> MELENYKQPVVLREDNCRRRRRMKPR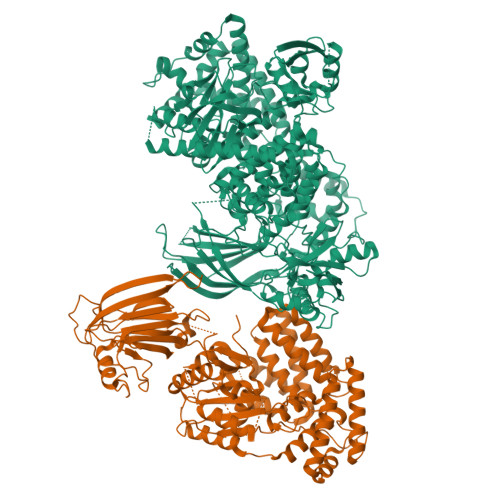SAAASLSSMELIPIEFVLPTSQRKCKSPETALLHVAGHGNVEQMKAQVWLRALETSVAADFYHRLGPHHFLLLYQKKGQWYEIYDKYQVVQTLDCLRYWKATHRSPGQIHLVQRHPPSEESQAFQRQLTALIGYDVTDVSNVHDDELEFTRRGLVTPRMAEVASRDPKLYAMHPWVTSKPLPEYLWKKIANNCIFIVIHRSTTSQTIKVSPDDTPGAILQSFFTKMAKKKSLMDIPESQSEQDFVLRVCGRDEYLVGETPIKNFQWVRHCLKNGEEIHVVLDTPPDPALDEVRKEEWPLVDDCTGVTGYHEQLTIHGKDHESVFTVSLWDCDRKFRVKIRGIDIPVLPRNTDLTVFVEANIQHGQQVLCQRRTSPKPFTEEVLWNVWLEFSIKIKDLPKGALLNLQIYCGKAPALSSKASAESPSSESKGKVQLLYYVNLLLIDHRFLLRRGEYVLHMWQISGKGEDQGSFNADKLTSATNPDKENSMSISILLDNYCHPIALPKHQPTPDPEGDRVRAEMPNQLRKQLEAIIATDPLNPLTAEDKELLWHFRYESLKHPKAYPKLFSSVKWGQQEIVAKTYQLLARREVWDQSALDVGLTMQLLDCNFSDENVRAIAVQKLESLEDDDVLHYLLQLVQAVKFEPYHDSALARFLLKRGLRNKRIGHFLFWFLRSEIAQSRHYQQRFAVILEAYLRGCGTAMLHDFTQQVQVIEMLQKVTLDIKSLSAEKYDVSSQVISQLKQKLENLQNSQLPESFRVPYDPGLKAGALAIEKCKVMASKKKPLWLEFKCADPTALSNETIGIIFKHGDDLRQDMLILQILRIMESIWETESLDLCLLPYGCISTGDKIGMIEIVKDATTIAKIQQSTVGNTGAFKDEVLNHWLKEKSPTEEKFQAAVERFVYSCAGYCVATFVLGIGDRHNDNIMITETGNLFHIDFGHILGNYKSFLGINKERVPFVLTPDFLFVMGTSGKKTSPHFQKFQDICVKAYLALRHHTNLLIILFSMMLMTGMPQLTSKEDIEYIRDALTVGKNEEDAKKYFLDQIEVCRDKGWTVQFNWFLHLVLGIKQGEKHSA;> GAGTMQPGATTCTEDRIQHALERCLHGLSLSRRSTSWSAGLCLNCWSLQELVSRDPGHFLILLEQILQKTREVQEKGTYDLLAPLALLFYSTVLCTPHFPPDSDLLLKAARTYHRFLTWPVPYCSICQELLTFIDAELKAPGISYQRLVRAEQGLSTRSHRSSTVTVLLLNPVEVQAEFLDVADKLSTPGPSPHSAYITLLLHAFQATFGAHCDLSGLHRRLQSKTLAELEAIFTETAEAQELASGIGDAAEARQWLRTKLQAVGEKAGFPGVLDTAKPGKLRTIPIPVARCYTYSWNQDSFDILQEILLKEQELLQPEILDDEEDEDEEDEEEDLDADGHCAERDSVLSTGSAASHASTLSLASSQASGPTLSRQLLTSFVSGLSDGVDSGYMEDIEESAYERPRRPGGHERRGHRRPGQKFNRIYKLFKSTSQMVLRRDSRSLEGSPDSGPPLRRAGSLCSPLDSPTLPPSRAQRSRSLPQPKLSPQLPGWLLAPASRHQRRRPFLSGDEDPKASTLRVVVFGSDRISGKVARAYSNLRRLENNRPLLTRFFKLQFFYVPVKRSRGTGTPTSPAPRSQTPPLPTDAPRHPGPAELGAAPWEESTNDISHYLGMLDPWYERNVLGLMHLPPEVLCQSLKAEPRPLEGSPAQLPILADMLLYYCRFAARPVLLQVYQTELTFITGEKTTEIFIHSLELGHSAATRAIKASGPGSKRLGIDGDREAVPLTLQIIYSKGAISGRSRWSNMEKLCTSVNLSKACRQQEELDSSTEALTLNLTEVVKRQTPKSKKGFNQISTSQIKVDKVQIIGSNSCPFAVCLDQDERKILQSVIRCEVSPCYKPEKSSLCPPPQRPSYPPAPATPDLCSLLCLPIMTFSGALP> FLVPPTVEQKTRPFTLPNLPLSSLSNSRAPLPISSMGISPDNVQSVQFQNGRCTLDGRLVGTTPVSLSHVAKIRGTSNGTVINLTELDGTPFHPFEGPAPIGFPDLGGCDWHINMTQFGHSSQTQYDVDTTPDTFVPHLGSIQANGIGSGNYVGVLSWISPPSHPSGSQVDLWKIPNYGSSITEATHLA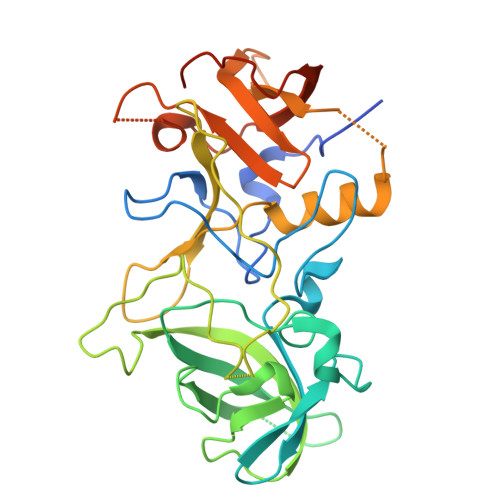PSVYPPGFGEVLVFFMSKMPGPGAYNLPCLLPQEYISHLASEQAPTVGEAALLHYVDPDTGRNLGEFKAYPDGFLTCVPNGASSGPQQLPINGVFVFVSWVSRFYQLKPVGTASSARGRLGLRR> TSVQNSPRLQQPQEQQQQQQQLSLKIKQLKLKRINELNNKLRKELSRERITASNACLTIINYTSNTKDYTLPELWGYPVAGSNHF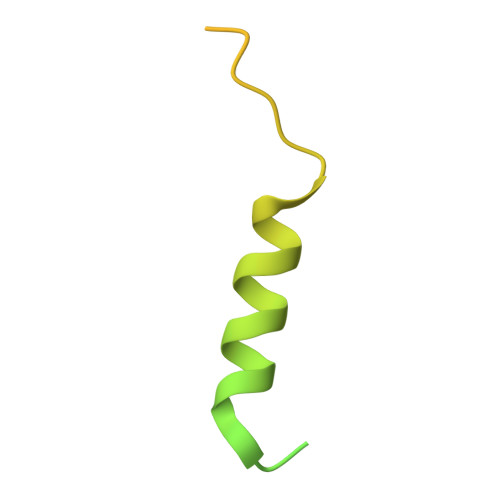IEGLKNAQKNSQMSNSNSVSSTLM>TVPKQIDIRNLIKELRNVEGVEEVHELHVWQLA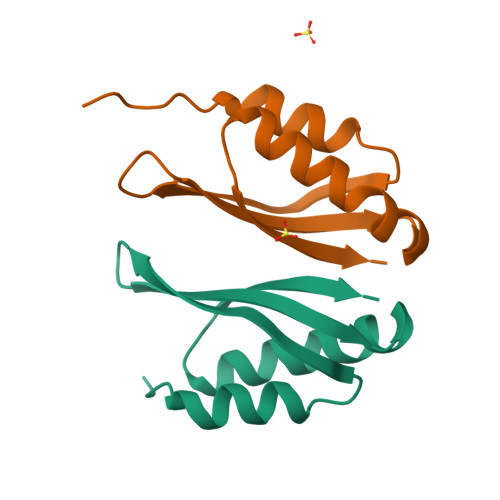GSRIIATAHIKCEDPTSYMEVAKTIKDVFHNHGIHATTIQPEF[2x]>[2x]GSHMAVQIGF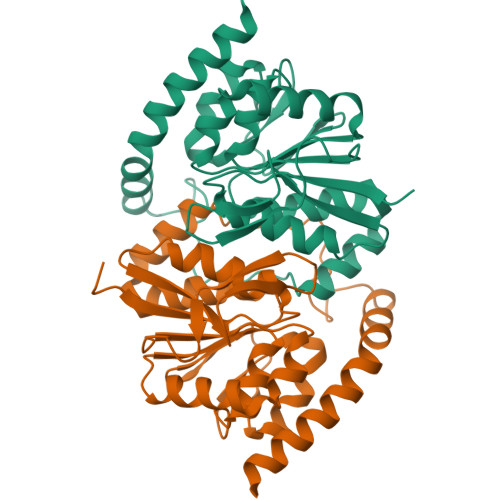LLFPEVQQLDLTGPHDVLASLPDVQVHLIWKEPGPVVASSGLVLQATTSFADCPPLDVICIPGGTGVGALMEDPQALAFIRQQAARARYVTSVCTGSLVLGAAGLLQGKRATTHWAYHELLAPLGAIPVHERVVRDGNLLTGAGITAGIDFALTLAAELFDAATAQRVQLQLEYAPAPPFNAGSPDTAPASVVQQARQRAADSLHKRREITLRAAARLAAG> APVWGCASTRGRSAEMEDASAAVPRFADVPVRLLASRRDLDALGLDADALRLPAHLFGVFDGHGGAEVANYCRERIHVVLSAALARLGKNLGEMGEVDMKEHWDDVFTKCFQRVDDEVSGRVTRVVNGGGEVRSEPVTAENVGSTAVVALVCSSHVVVANCGDSRIVLCRGKEPVALSIDHKPDR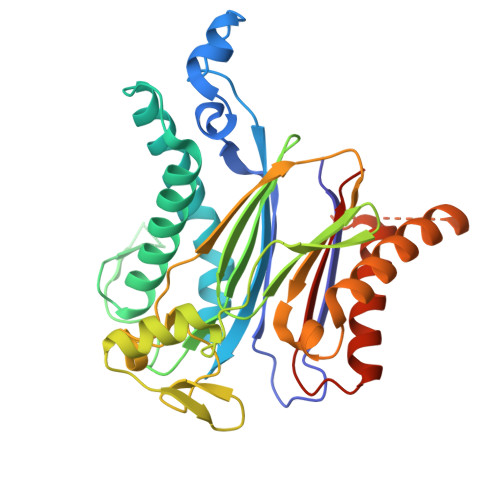KDERARIEAQGGKVIQWNGYRVLGVLAMSRSIGDRYLKPFVIPKPEVMVVPRAKDDDCLILASDGLWDVVSNEEACKVARRQILLWHKNNGAASPLSDEGEGSTDPAAQAAADYLMRLALKKGSEDNITVIVVDLKPRKKLKN>PGIHSGRTRVGKYELGRTLGEGTFAKVKFARNVENGDNVAIKVIDKEKVLKNKMIAQIKREISTMKLIKHPNVIRMFEVMASKTKIYFVLEFVTGGELFDKISSNGRLKEDEARKYFQQLINAVDYCHSRGVYHRDLKPENLLLDANGALKVSDFGLSALPQQVREDGLLHDTCGTPNYVAPEVINNKGYDGAKADLWSCGVILFVLMAGYLPFEDSNLTSLYKKIFKAEFTCPPWFSASAKKLIKRILDPNPATRITFAEVIENEWFKKGYKAPKFENADVSLDDVDAIFDDSGESKNLVVERREEGLKTPVTMNAFELISTSQGLNLGSLFEKQMGLVKRKTRFTSKSSANEIVTKIEAAAAPMGFDVKTNNY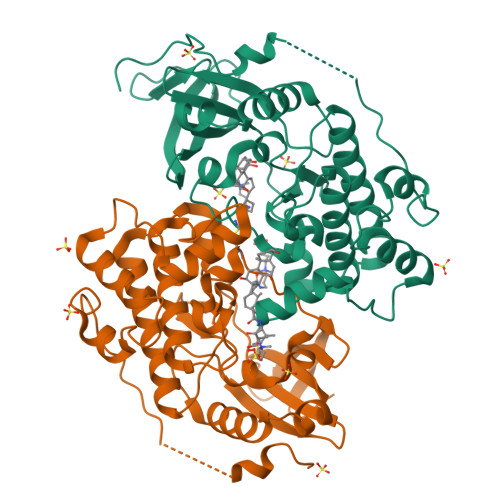KMKLTGEKSGRKGQLAVATEVFQVAPSLYMVEMRKSGGDTLEFHKFYKNLTTGLKDIVWKTIDEEKEEGTDGGGTNGAMANRTIAKQST[4x]methyl (2~{R})-3-(4-hydroxyphenyl)-2-[(4-hydroxyphenyl)methyl]-4-oxidanyl-5-oxidanylidene-furan-2-carboxylate 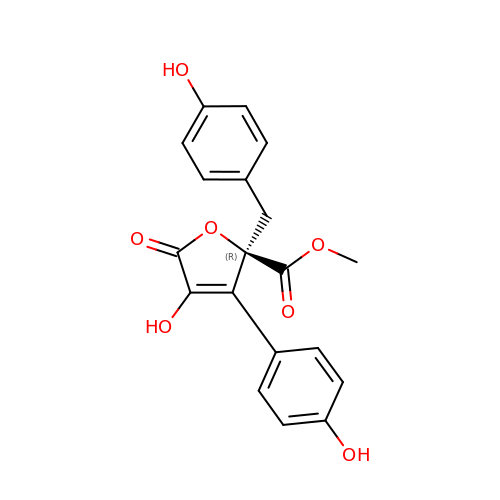| C19 H16 O7 | AEKPZNDJHWFONI-LJQANCHMSA-N>MNPYERGPNPTDALLEARSGPFSVSEENVSRLSASGFGGGTIYYPRENNTYGAVAISPGYTGTEASIAWLGERIASHGFVVITIDTITTLDQPDSRAEQLNAALNHMINRASSTVRSRIDSSRLAVMGHSMGGGGSLRLASQRPDLKAAIPLTPWHLNKNWSSVTVPTLIIGADLDTIAPVATSAKPIYNSLPSSISKAYLELDGATHFAPNIPNKIIGKYSVAWLKRFVDNDTRYTQFLCPGPRDGLFGEVEEYRSTCPF[2x]

Cutinase is an esterase that belongs to the α/β-hydrolase superfamily and primarily hydrolyzes cutin from plants. Unlike lipases, cutinases lack the active site-covering lid structure such that the substrate-binding cleft is exposed and directly accessible from bulk solution. In addition, the substrate-binding site is more expansive in cutinases compared to esterases, benefiting the binding of bulkier macromolecules. In this work, we investigate the PBAT hydrolysis potency of cutinases and PET-degrading enzymes, and find that cutinases outcompete other reported enzymes.

In order to understand the mechanism of action of the DM variant of cutinase, we aimed to solve their crystal structures and eventually obtained crystal structures of the apo-form and substrate analog complex of TfCut-DM. The crystal structure of apo-TfCut-DM was solved to 2.20 Å resolution and it contains two polypeptide chains in an asymmetric unit. Superimposing the structure with the previously reported WT TfCut yields an RMSD value of 0.255 Å for all Cα carbons, indicating that the overall structure is maintained. The crystal structure of TfCut-DM shows a classical α/β-hydrolase in which nine β-sheets are sandwiched by eight α-helices on both sides. The catalytic triad residues, S170, D216, and H248, are located in the loop regions between α5 and β5, α6 and β7, and α7 and β8, respectively. The DM residues, S224 and I228, are located below the catalytic triad. It is worth noting that the side-chain of W195 in TfCut-DM switches from C-type conformation in the WT TfCut structure to B-type conformation according to the assignment in the previous publication. Note that W195 only exhibits B-type in the reported TfCut-DM crystal, while the corresponding residue in the previously solved IsPETase crystal shows A-, B-, and C-type conformations. Since the Trp conformation is determined by the two-residue located beneath the Trp, we presumed that W195 can still wobble in the apo-form, though alternate conformations were not captured in this crystal.>[4x]CGCGAAUUAGCG

GNA comprises an acyclic, three-carbon backbone with a single stereocenter and currently constitutes the simplest known nucleic acid self-pairing system with a phosphodiester backbone. Further evaluation of GNA crystal structures pointed towards a global structure of the (S)-isomer which closely mimics the backbone of an A-form helix, likely explaining the preference for cross-pairing with RNA but not DNA. A reexamination of published GNA homoduplex crystal structures, along with a novel structure containing a single (S)-GNA-A residue in duplex RNA, indicated that GNA nucleotides universally adopt a rotated nucleobase orientation within all duplex contexts. Such an orientation strongly affects GNA-C and GNA-G but not GNA-A or GNA-T pairing in GNA/RNA heteroduplexes.

To expand upon our previous structural work on the behavior of pyrimidine GNA nucleotides ((S)-GNA-T) in RNA duplexes, we determined the crystal structure of 5′-CGCGAA-BrU-UAGCG-3′ (A= (S)-GNA-A; BrU = 5-bromo-Uridine) at a resolution of 1.78 Å. This sequence was chosen since it has previously provided high quality structures (RNA with or without modified nucleotides) and resulted in the highest quality diffracting crystals of an RNA duplex containing GNA-A. The modified dodecamer crystallizes in space group P32 with two independent duplexes per crystallographic asymmetric unit along with 156 water molecules. All four GNA-A residues pair with uridine in the reverse Watson–Crick mode. The adenine nucleobases of GNA project their N6 and N7 atoms into the minor groove and form two H-bonds with uridine: [gA]N6-H…O2[rU] and [gA]N1…H-N3[rU]. The structure confirms that GNA does not alter its hallmark inverted base orientation inside RNA and appears unable to adapt to the standard Watson–Crick pairing mode, thereby precluding the formation of three H-bonds in mixed GNA/RNA G:C pairs. Rather, the structurally constrained backbone in GNA forces a change in the nucleobase orientation where the base is projected into the duplex from the side of the major instead of minor groove, resulting in the formation of reverse Watson–Crick pairs opposite RNA similar to what is observed in parallel duplexes of RNA or DNA. In this report we show that rotation of the base orientation in GNA nucleotides, first observed in an RNA duplex structure containing GNA-T, is common to all GNA nucleotides, whether present in GNA homoduplexes or GNA/RNA heteroduplex contexts. Although reverse Watson–Crick pairing does not have a large impact on cross-pairing of GNA-A or -T with complementary RNA nucleotides, it strongly disrupts the ability of GNA-C or -G to form a complementary base pair with RNA. The right-handed and negatively inclined (S)-GNA strand pairs stably with RNA, but does not tolerate G:C pairs because they feature only two H-bonds (reverse Watson–Crick) rather than three in the standard Watson–Crick pairing mode, are sheared, and result in less optimal stacking.>[2x]SNAMPKRSKEDTEITIQKIMDAVVDQLLRLGYDKMSYTTLSQQTGVSRTGISHHFPKKTDFTAALDGRIFKMFIEHLEFEKGLDAFSQSWIKALEDSEFLAILRLLFHHIVTSESAHEFA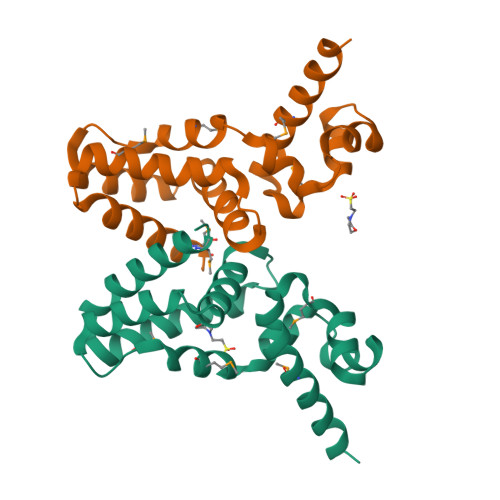ANGIDRLYKMVESQFGSGGDKELEWLIGRSLIQMSK>MTALFDLTGKTALVTGSARGLGFAYAEGLAAAGARVILNDIRATLLAESVDTLTRKGYDAHGVAFDVTDELAIEAAFSKLDAEGIHVDILINNAGIQYRKPMVELELENWQKVIDTNLTSAFLVSRSAAKRMIARNSGGKIINIGSLTSQAARPTVAPYTA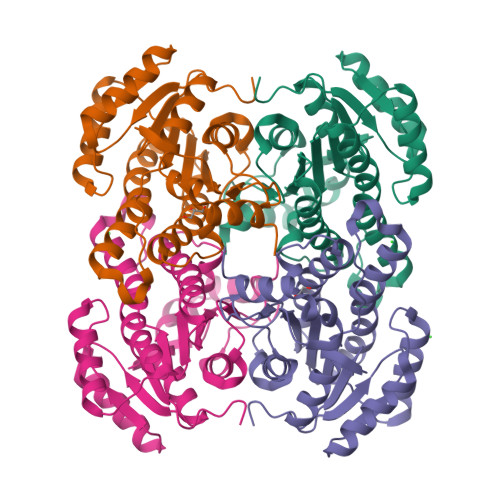AKGGIKMLTCSMAAEWAQFNIQTNAIGPGYILTDMNTALIEDKQFDSWVKSSTPSQRWGRPEELIGTAIFLSSKASDYINGQIIYVDGGWLAVL[4x]> LTKINETESEKLLSLEDTLHERVIGQKDAVNSISKAVRRARAGLKDPKRPIGSFIFLGPTGVGKTELARALAESMFGDDDAMIRVDMSEFMEKHAVSRLVGAPPGYVGHDDGGQLTEKVRRKPY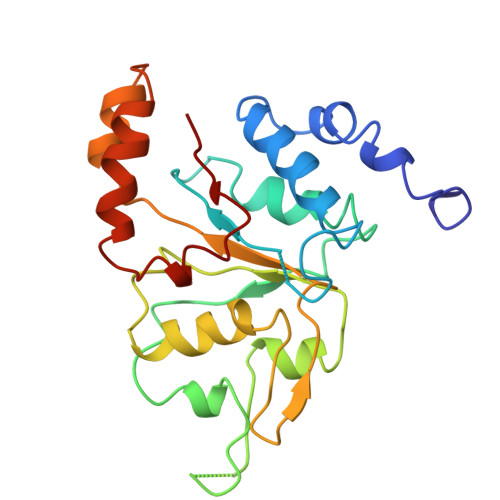SVILFDEIEKAHPDVFNILLQVLDDGHLTDTKGRTVDFRNTIIIMTSNVGAQELQDQRFAGFGGSSDGQDYETIRKTMLKELKNSFRPEFLNRVDDIIVFH> ADLGSKNLKSPQKVEVDIIDDNFILRWNRSDESVGNVTFSFDYQKTGMDNWIKLSGCQNITSTKCNFSSLKLNVYEEIKLRIRAEKENTSSWYEVDSFTPFRKAQIGPPEVHLEAEDKAIVIHISPGTKDSVMWALDGLSFTYSLVIWKNSSGVEERIENIYSRHKIYKLSPETTYCLK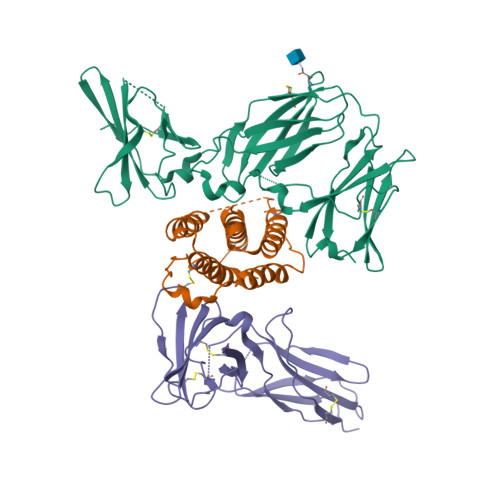VKAALLTSWKIGVYSPVHCIKTTVENELPPPENIEVSVQNQNYVLKWDYTYANMTFQVQWLHAFLKRNPGNHLYKWKQIPDCENVKTTQCVFPQNVFQKGIYLLRVQASDGNNTSFWSEEIKFDTEIQAFLLPPVFNIRSLSDSFHIYIGAPKQSGNTPVIQDYPLIYEIIFWENTSNAERKIIEKKTDVTVPNLKPLTVYCVKARAHTMDEKLNKSSVFSDAVCEKTKPGNTSK;> ADPLGCDLPQNHGLLSRNTLVLLHQMRRISPFLCLKDRRDFRFPQEMVKGSQLQKAHVMSVLHEMLQQIFSLFHTERSSAAWQMTLLDQLHTGLHQQLQHLETCLLQVVGEGESAGAISSPALTLRRYFQGIRVYLKEKKYSDCAWEVVRMEIMKSLFLSTNMQERLRSKDRDLGSS;> YTDESCTFKISLRNFRSILSWELKNHSIVPTHYTLLYTIMSKPEDLKVVKNCANTTRSFCDLTDEWRSTHEAYVTVLEGFSGNTTLFSCSHNFWLAIDMSFEPPEFEIVGFTNHINVMVKFPSIVEEELQFDLSLVIEEQSEGIVKKHKPEIKGNMSGNFTYIIDKLIPNTNYCVSVYLEHSDEQAVIKSPLKCTLLPP>MAVVPASLSGQDVGSFAYLTIKDRIPQILTKVIDTLHRHKSEFFEKHGEEGVEAEKKAISLLSKLRNELQTDKPFIPLVEKFVDTDIWNQYLEYQQSLLNESDGKSRWFYSPWLLVECYMYRRIHEAIIQSPPIDYFDVFKESKEQNFYGSQESIIALCTHLQQLIRTIEDLDENQLKDEFFKLLQISLWGNKCDLSLSGGESSSQNTNVLNSLEDLKPFILLNDMEHLWSLLSNCKKTREKASATRVYIVLDNSGFELVTDLILADFLLSSELATEVHFYGKTIPWFVSATTIHDFNWLIEQVKHSNHKWMSKCGADWEEYIKMGKWVYHNHIFWTLPHEYCAMPQVAPDLYAELQKAHLILFKGDLNYRKLTGDRKWEFSVPF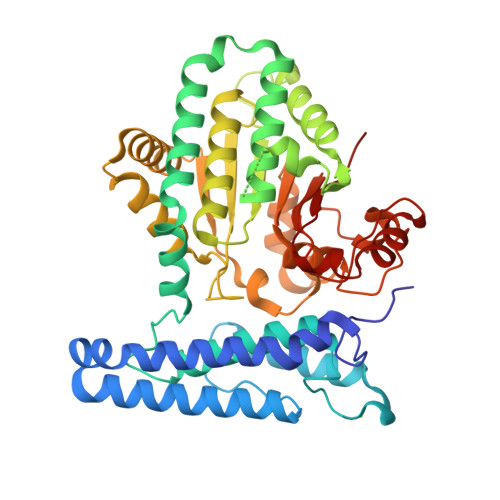HQALNGFHPAPLCTIRTLKAEIQVGLQPGQGEQLLASEPSWWTTGKYGIFQYDGPL[2x]> ASMDNYIYSIAHQLYEMYLQDEDAFHSKRDYPHKKVFTELQKLRKIFFPDFFMKHQKITESHIASELTKLVDYIKDSVTAYNDELFAHQCVMAILEKLPSIKRTLKTDLIAAYAGDPAAPGLSLIIRCYPGFQAVIVYRIAHVLYECGERYYCREMMESVHSYTSIDIHPGASIKGHFFIDHGVGVVIGETAIIGEWCRIYQSVTLGAMHFQEEGGVIKRGTKRHPTVGDYVTIGTGAKVLGNIIVGSHVRIGANCWIDRDVDSNQTVYISEHPTHFVKPCTTK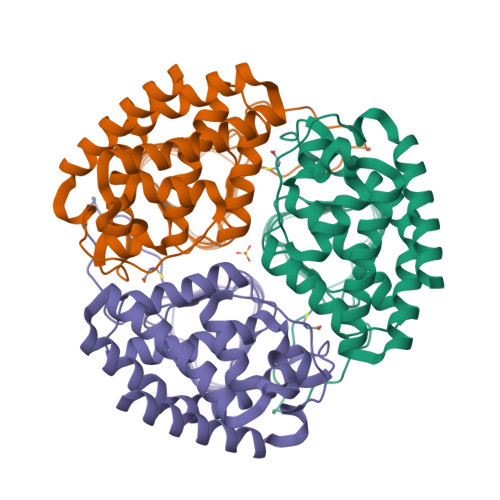GMKNDTEIIAIIPSSPLANSPSILEHHHHHH>MSAKAISEQTGKELLYKFICTTSAIQNRFKYARVTPDTDWARLLQDHPWLLSQNLVVKPDQLIKRRGKLGLVGVNLTLDGVKSWLKPRLGQEATVGKATGFLKNFLIEPFVPHSQAEEFYVCIYATREGDYVLFHHEGGVDVGDVDAKAQKLLVGVDEKLNPEDIKKHLLVHAPEDKKEILASFISGLFNFYEDLYFTYLEINPLVVTKDGVYVLDLAAKVDATADYICKVKWGDIEFPPPFGREAYPEEAYIADLDAKSGASLKLTLLNPKGRIWTMVAGGGASVVYSDTICDLGGVNELANYGEYSGAPSEQQTYDYAKTILSLMTREKHPDGKILIIGGSIANFTNVAATFKGIVRAIRDYQGPLKEHEVTIFVRRGGPNYQEGLRVMGEVGKTTGIPIHVFGTETHMTAIVGMALGHRPIPNQPPTAAHTANFLLNASGSTSTPAPSRTASFSESRADEVAPAKKAKPAMPQDSVPSPRSLQGKSTTLFSRHTKAIVWGMQTRAVQGMLDFDYVCSRDEPSVAAMVYPFTGDHKQKFYWGHKEILIPVFKNMADAMRKH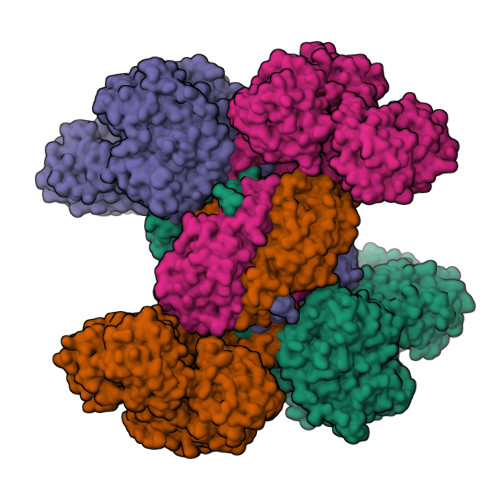PEVDVLINFASLRSAYDSTMETMNYAQIRTIAIIAEGIPEALTRKLIKKADQKGVTIIGPATVGGIKPGCFKIGNTGGMLDNILASKLYRPGSVAYVSRSGGMSNELNNIISRTTDGVYEGVAIGGDRYPGSTFMDHVLRYQDTPGVKMIVVLGEIGGTEEYKICRGIKEGRLTKPIVCWCIGTCATMFSSEVQFGHAGACANQASETAVAKNQALKEAGVFVPRSFDELGEIIQSVYEDLVANGVIVPAQEVPPPTVPMDYSWARELGLIRKPASFMTSICDERGQELIYAGMPITEVFKEEMGIGGVLGLLWFQKRLPKYSCQFIEMCLMVTADHGPAVSGAHNTIICARAGKDLVSSLTSGLLTIGDRFGGALDAAAKMFSKAFDSGIIPMEFVNKMKKEGKLIMGIGHRVKSINNPDMRVQILKDYVRQHFPATPLLDYALEVEKITTSKKPNLILNVDGLIGVAFVDMLRNCGSFTREEADEYIDIGALNGIFVLGRSMGFIGHYLDQKRLKQGLYRHPWDDISYVLPEHMSM[4x]>[2x]SWQAYTDNLIGTGKVDKAVIYSRAGDAVWATSGGLSLQPNEIGEIVQGFDNPAGLQSNGLHIQGQKFMLLRADDRSIYGRHDAEGVVCVRTKQTVIIAHYP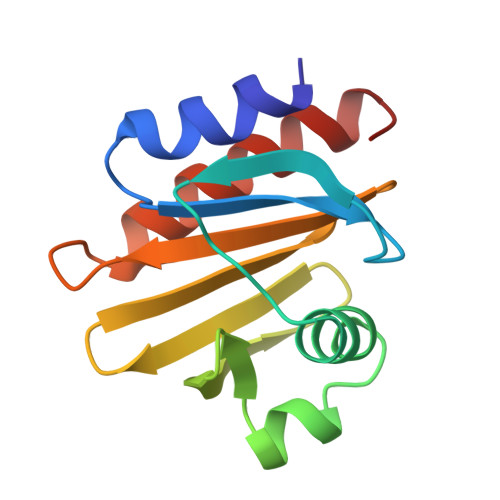PTVQAGEATKIVEQLADYLIGVQY2-{2-[(1-aminoisoquinolin-6-yl)carbamoyl]-6-methoxypyridin-3-yl}-5-{[(2S)-1-hydroxy-3,3-dimethylbutan-2-yl]carbamoyl}benzoic 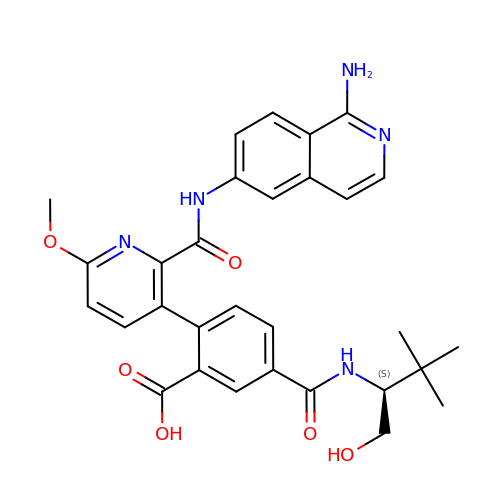acid | C30 H31 N5 O6 | GCBXPOHPNDVIFD-HSZRJFAPSA-N>MNTKYNKEFLLYLAGFVDGNGSIIAQIKPNQSYKFKHQLSLTFQVTQKTQRRWFLDKLVDEIGVGYVRDRGSVSDYILSEIKPLHNFLTQLQPFLKLKQKQANLVLKIIEQLPSAKESPDKFLEVCTWVDQIAALNDSKTRKTTSETVRAVLDSLS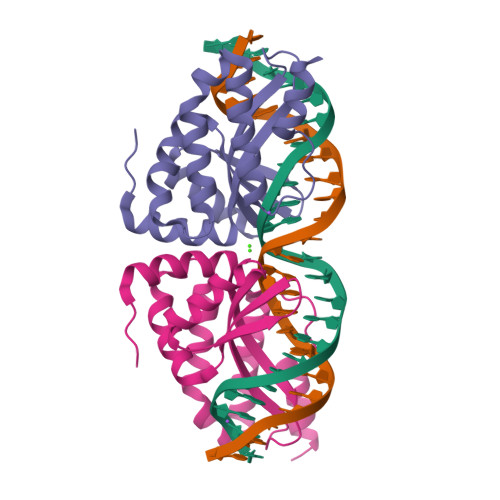EKKKSSP[2x]Pseudomonas aeruginosa (Pae) SutA adapts bacteria to hypoxia and nutrition-limited environment during chronic infection by increasing transcription activity of an RNA polymerase (RNAP) holoenzyme comprising the stress-responsive σ factor σS (RNAP-σS). To understand the molecular mechanism of SutA activation, here we determined cryo-EM structures of RNAP-σS holoenzyme at 4.1 Å, SutA-bound RNAP-σS holoenzyme at 3.1 Å (SutA-RNAP-σS, open lobe) and 3.9 Å (SutA-RNAP-σS, closed lobe), and SutA-bound RNAP-σS promoter open complex (SutA-σS-RPo) at 5.8 Å. The structures reveal that SutA pinches RNAP-β protrusion with its RNAP-binding domain and wedges RNAP-β lobe open to facilitate promoter unwinding with its wedge loop and N-terminal D/E-rich region. SutA anchors RNAP-β protrusion through its RBD and wedges open β lobe through its wedge loop to facilitate RPo formation.

As no structural information is available for bacterial RNAP- σS holoenzyme, we reconstituted Pae RNAP-σS holoenzyme and determined its structure through the single-particle cryo-EM approach. Focused 3D classification resulted in a single group of RNAP-σS holoenzyme particles, from which a cryo-EM map of the RNAP-σS holoenzyme was reconstituted at resolution 4.1 Å. The cryo-EM map shows strong continuous signals for all domains of σS except for σS1.1. The weak fractionated map signal of σS1.1 domain in the main cleft of RNAP suggests its conformational heterogeneity and low occupancy. We compared the binding affinity of Pae RNAP core enzyme towards σA1.1 or σS1.1 by using a fluorescence polarization assay. The results showed that the σA1.1 domain binds RNAP core enzyme with a Kd value of 220 nM, but the interaction between σS1.1 domain and RNAP core enzyme is barely detectable under the same experimental condition, indicating that σS1.1 binds to RNAP core enzyme much weaker compared with σA1.1. Structure superimposition of the SutA-RNAP-σS (open lobe) and RNAP-σS holoenzyme complexes shows differences in RNAP-β lobe conformation and main cleft width. In sharp contrast, there exists substantial steric clashes between the modeled dsDNA and RNAP in the RNAP-σS holoenzyme. RNAP-β lobe of RNAP holoenzyme is in rapid equilibrium between open and closed conformation but with preference on being closed.

>[2x]MGHHHHHHHHHHMQSSVNEFLTPRHIDVQVVSQTRAKITLEPLERGFGHTLGNALRRILLSSMPGCAVVEAEIDGVLHEYSAIEGVQEDVIEILLNLKGLAIKLHGRDEVTLTLAKKGSGVVTAADIQLDHDVEIINGDHVIANLADNGALNMKLKVARGRGYEPADARQSDEDESRSIGRLQLDASFSPVRRVSYVVENARVEQRTNLDKLVLDLETNGTLDPEEAIRRAATILQQQLAAFVDLKGDSEPVVEEQEDEIDPILLRPVDDLELTVRSANCLKAENIYYIGDLIQRTEVELLKTPNLGKKSLTEIKDVLASRGLSLGMRLDNWPPASLKKDDKATA;> MGMAYSYTEKKRIRKDFSKLPDVMDVPYLLAIQLDSYREFLQAGATKEQFRDVGLHAAFKSVFPIISYSGNAALEYVGYRLGEPAFDVKECVLRGVTFAVPLRVKVRLIIFDRESSNKAIKDIKEQEVYMGEIPLMTENGTFIINGTERVIVSQLHRSPGVFFDHDRGKTHSSGKLLYSARIIPYRGSWLDFEFDPKDCVFVRIDRRRKLPASVLLRALGYSTEEILNAFYATNVFHIKGETLNLELVPQRLRGEVASIDIKDGSGKVIVEQGRRITARHINQLEKAGVSQLEVPFDYLIGRTIAKAIVHPATGEIIAECNTELTLDLLAKVAKAQVVRIETLYTNDIDCGPFISDTLKIDNTSNQLEALVEIYRMMRPGEPPTKEAAETLFGNLFFSAERYDLSAVGRMKFNRRIGRTEIEGPGVLSKEDIIDVLKTLVDIRNGKGIVDDIDHLGNRRVRCVGEMAENQFRVGLVRVERAVKERLSMAESEGLMPQDLINAKPVAAAIKEFFGSSQLSQFMDQNNPLSEITHKRRVSALGPGGLTRERAGFEVRDVHPTHYGRVCPIETPEGPNIGLINSLATYARTNKYGFLESPYRVVKDSLVTDEIVFLSAIEEADHVIAQASATLNEKGQLVDELVAVRHLNEFTVKAPEDVTLMDVSPKQVVSVAASLIPFLEHDDANRALMGSNMQRQAVPTLRADKPLVGTGMERNVARDSGVCVVARRGGVIDSVDASRVVVRVADDEVETGEAGVDIYNLTKYTRSNQNTCINQRPLVSKGDVVARGDILADGPSTDMGELALGQNMRVAFMPWNGFNFEDSICLSERVVQEDRFTTIHIQELTCVARDTKLGPEEITADIPNVGEAALNKLDEAGIVYVGAEVQAGDILVGKVTPKGETQLTPEEKLLRAIFGEKASDVKDTSLRVPTGTKGTVIDVQVFTRDGVERDSRALSIEKMQLDQIRKDLNEEFRIVEGATFERLRAALVGAKAEGGPALKKGTEITDDYLDGLERGQWFKLRMADDALNEQLEKAQAYISDRRQLLDDKFEDKKRKLQQGDDLAPGVLKIVKVYLAIKRRIQPGDKMAGRHGNKGVVSVIMPVEDMPHDANGTPVDIVLNPLGVPSRMNVGQILETHLGLAAKGLGEKINRMLEEQRKVAELRKFLHEIYNEIGGREENLDELGDNEILALAKNLRGGVPMATPVFDGAKEREIKAMLKLADLPESGQMRLFDGRTGNQFERPTTVGYMYMLKLNHLVDDKMHARSTGSYSLVTQQPLGGKAQFGGQRFGEMEVWALEAYGAAYTLQEMLTVKSDDVNGRTKMYKNIVDGDHRMEAGMPESFNVLIKEIRSLGIDIELETE;> MLKDLLNLLKNQGQIEEFDAIRIGLASPEMIRSWSFGEVKKPETINYRTFKPERDGLFCAKIFGPVKDYECLCGKYKRLKHRGVICEKCGVEVALAKVRRERMGHIELASPVAHIWFLKSLPSRIGLLLDMTLRDIERVLYFESYVVIDPGMTTLEKGQLLNDEQYFEALEEFGDDFDARMGAEAVHELLNAIDLEHEIGRLREEIPQTNSETKIKKLSKRLKLMEAFQGSGNKPEWMVLTVLPVLPPDLRPLVPLDGGRFATSDLNDLYRRVINRNNRLKRLLDLAAPDIIVRNEKRMLQEAVDALLDNGRRGRAITGSNKRPLKSLADMIKGKQGRFRQNLLGKRVDYSGRSVITVGPTLRLHQCGLPKKMALELFKPFIFGKLEGRGMATTIKAAKKMVERELPEVWDVLAEVIREHPVLLNRAPTLHRLGIQAFEPVLIEGKAIQLHPLVCAAYNADFDGDQMAVHVPLTLEAQLEARALMMSTNNILSPANGEPIIVPSQDVVMGLYYMTREAINAKGEGMAFADLQEVDRAYRSGQASLHARVKVRINEKIKGEDGQLTANTRIVDTTVGRALLFQVVPAGLPFDVVNQSMKKKAISKLINHCYRVVGLKDTVIFADQLMYTGFAYSTISGVSIGVNDFVIPDEKARIINAATDEVKEIESQYASGLVTQGEKYNKVIDLWSKANDEVSKAMMANLSKEKVVDREGKEVDQESFNSMYMMADSGARGSAAQIRQLAGMRGLMAKPDGSIIETPITANFREGLNVLQYFISTHGARKGLADTALKTANSGYLTRRLVDVAQDLVVTEIDCGTEHGLLMSPHIEGGDVVEPLGERVLGRVIARDVFKPGSDEVIVPAGTLIDEKWVDFLEVMSVDEVVVRSPITCETRHGICAMCYGRDLARGHRVNIGEAVGVIAAQSIGEPGTQLTMRTFHIGGAASRTSAADNVQVKNGGTIRLHNLKHVVRADGALVAVSRSGELAVADDFGRERERYKLPYGAVISVKEGDKVDPGAIVAKWDPHTHPIVTEVDGTVAFVGMEEGITVKRQTDELTGLTNIEVMDPKDRPAAGKDIRPAVKLIDAAGKDLLLPGTDVPAQYFLPANALVNLTDGAKVSIGDVVARIPQETSKTRDITGGLPRVADLFEARRPKEPSILAEISGTISFGKETKGKRRLVITPNDGSDPYEELIPKWRHLNVFEGEQVNRGEVISDGPSNPHDILRLLGVSSLAKYIVNEIQDVYRLQGVKINDKHIETILRQMLRKVEVSESGDSSFIKGDQVELTQVLEENEQLGTEDKFPAKYERVLLGITKASLSTESFISAASFQETTRVLTEAAVTGKRDFLRGLKENVVVGRLIPAGTGLAYHSERKRQRDLGKPQRVSASEAEAALTEALNSSGNGSGSWSHPQFEK;> MARVTVEDCLDNVDNRFELVMLATKRARQLATGGKEPKVAWENDKPTVVALREIASGLVDENVVQQEDIVEDEPLFAAFDDEANTEAL;> GAMGMALKKEGPEFDHDDEVLLLEPGIMLDESSADEQPSPRATPKATTSFSSKQHKHIDYTRALDATQLYLNEIGFSPLLTPEEEVHFARLAQKGDPAGRKRMIESNLRLVVKIARRYVNRGLSLLDLIEEGNLGLIRAVEKFDPERGFRFSTYATWWIRQTIERAIMNQTRTIRLPIHVVKELNVYLRAARELTHKLDHEPSPEEIANLLEKPVAEVKRMLGLNERVTSVDVSLGPDSDKTLLDTLTDDRPTDPCELLQDDDLSESIDQWLTELTDKQREVVIRRFGLRGHESSTLEEVGQEIGLTRERVRQIQVEALKRLREILEKNGLSSDALFQ> ASSLPPNALKPAFGPPDKVAAQKFKESLMATEKHAKDTSNMWVKISVWVALPAIALTAVNTYFVEKEHAEHREHLKHVPDSEWPRDYEFMNIRSKPFFWGDGDKTLFWNPVVNRHIEHDDG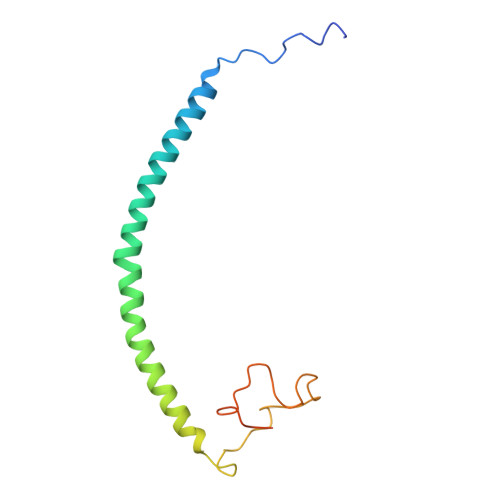ARGSHHHHHH>GSHGMKVVIAGRPNAGKSSLLNALAGREAAIVTDIAGTTRDVLREHIHIDGMPLHIIDTAGLREASDEVERIGIERAWQEIEQADRVLFMVDGTTTDAVDPAEIWPEFIARLPAKLPITVVRNKADITGETLGMSEVNGHALIRLSARTGEGVDVLRNHLK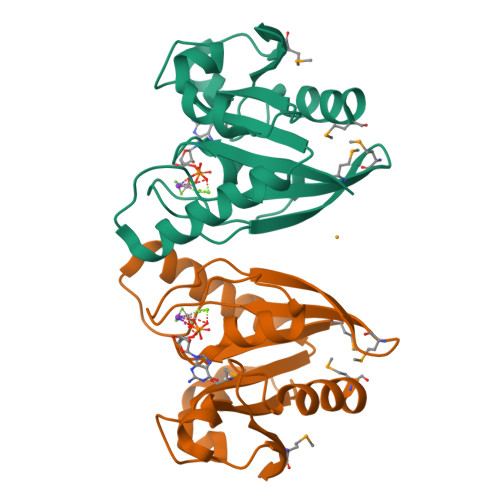QSMGFDTNMEG[4x]> RQVIVPVCMPKIHYSPLKTGLCYDVRMRYHAKIFTSYFEYIDPHPEDPRRIYRIYKI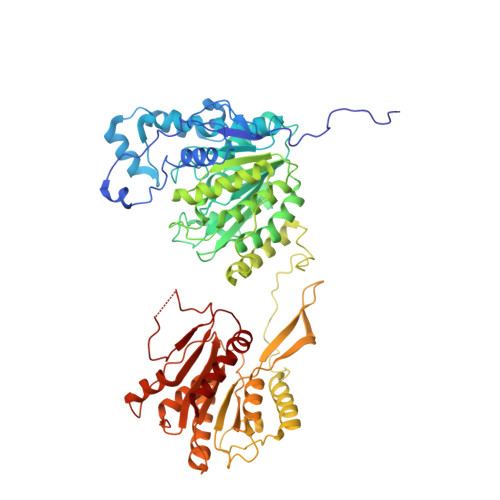LAENGLINDPTLSGVDDLGDLMLKIPVRAATSEEILEVHTKEHLEFIESTEKMSREELLKETEKGDSVYFNNDSYASARLPCGGAIEACKAVVEGRVKNSLAVVRPPGHHAEPQAAGGFCLFSNVAVAAKNILKNYPESVRRIMILDWDIHHGNGTQKSFYQDDQVLYVSLHRFEMGKYYPGTIQGQYDQTGEGKGEGFNCNITWPVGGVGDAEYMWAFEQVVMPMGREFKPDLVIISSGFDAADGDTIGQCHVTPSCYGHMTHMLKSLARGNLCVVLEGGYNLDAIARSALSVAKVLIGEPPDELPDPLSDPKPEVIEMIDKVIRLQSKYWNCFRRRHANSGCNFNEPLNDSIISKNFPLQKAIRQQQQHYLSDEFNFVTLPLVSMDLPDNTVLCTPNISESNTIIIVVHDTSDIWAKRNVISGTIDLSSSVIIDNSLDFIKWGLDRKYGIIDVNIPLTLFEPDNYSGMITSQEVLIYLWDNYIKYFPSVAKIAFIGIGDSYSGIVHLLGHRDTRAVTKTVINFLGDKQLKPLVPLVDETLSEWYFKNSLIFSNNSHQCWKENESRKPRKKFGRVLRCDTDGLNNIIEERFEEATDFILDSFE> ICSGPQNLAQELKAIGDQLQELQKKLIQGPNISQPRPLLTIETPRHLGEQLNARRKELGIDLYTLELQTGISTSTLKRLFKDP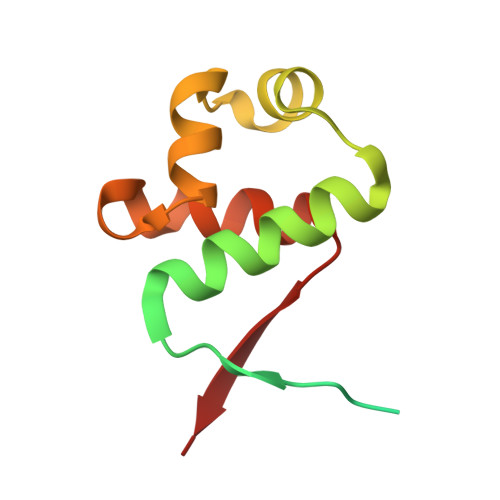EQVKFGSVFAVANVLGVKLCIGE>[2x]MLEKVETFDMNRVIDEFDEMTRNAHQV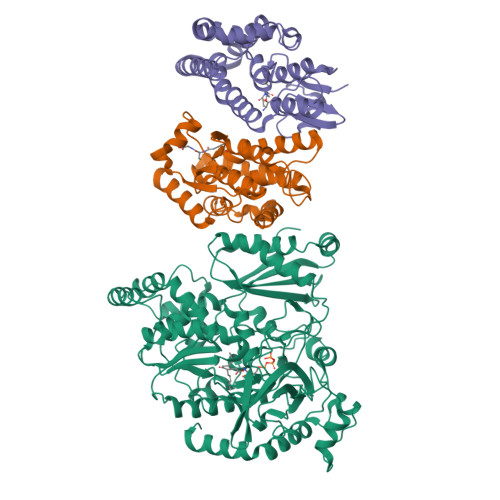QKQTLKEILLKNQSAIYLQNCGLNGNATDPEEAFKSMVPLVTDVELEPYIKRMVDGDTSPILTGHPVPAISLSSGTSQGRPKFIPFTDELMENTLQLFRTAFAFRNRDFPIDDNGKALQFIFSSKQYISTGGVPVGTATTNVYRNPNFKAGMKSITSPSCSPDEVIFSPDVHQALYCHLLSGILFRDQVQYVFAVFAHGLVHAFRTFEQVWEEIVTDIKDGVLSNRITVPSVRTAMSKLLTPNPELAETIRTKCMSLSNWYGLIPALFPNAKYVYGIMTGSMEPYVPKLRHYAGDLPLVSHDYGSSEGWIAANVTPRLSPEEATFAVIPNLGYFEFLPVSETGEGEEKPVGLTQVKIGEEYEVVITNYAGLYRYRLGDVVKVIGFYNNTPQLKFICRRNLILSINIDKNTERDLQLSVESAAKRLSEEKIEVIDFSSYIDVSTDPGHYAIFWEISGETNEDVLQDCCNCLDRAFIDAGYVSSRKCKTIGALELRVVAKGTFRKIQEHFLGLGSSAGQFKMPRCVKPSNAKVLQILCENVVSSYFSTAF;>HHHHHHMANLPILLDYWPSMFGMRARVALREKGVEFEYREEDFSNKSPLLLQSNPIHKKIPVLVHNGKPVCESLNVVQYVDEAWPEKNPFFPSDPYGRAQARFWADFVDKKFTDAQFKVWGKKGEEQEAGKKEFIEAVKILESELGDKPYFGGDSFGYVDISLITFSSWFQAYEKFGNFSIESESPKLIAWAKRCMEKESVSKSLPDSEKIVAYAAEYRKNNL[4x]>[2x]GSMAEVGSKSVLFVCLGNICRSPIAEAVFRKLVTDEKVSDNWRIDSAATSTYEVGNPPDYRGQNCMRKHGIHMQHIARQITKEDFATFDYILCMD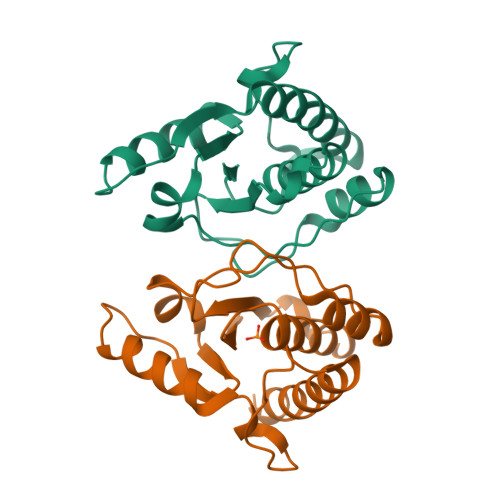ESNLRDLNRKSNQVKNCKAKIELLGSYDPQKQLIIEDPYYGNDSDFEVVYQQCLRCCKAFLEKTY We identify a hitherto uncharacterized protein factor that we term UBP (ucm-binding protein) that interacts sequence-specifically with the ucm and determine the structure of the protein both in isolation and when bound to DNA. UBP is a highly abundant protein, and we reveal that it plays a role akin to bacterial nucleoid-associated proteins with over 300 binding sites on the Sulfolobus chromosome. Importantly, UBP interacts with the N-terminal domains of MCM. Taken together, our data provide evidence that UBP functions as a general nucleoid-associated protein that plays a key role in facilitating the egress of the MCM replicative helicase from DNA replication origins.

Next, we solved the structure of UBP bound to DNA containing a ucm site to 1.8 Å resolution. We attempted crystallization with a range of sizes of DNA molecule; the only construct that yielded crystal formation was a 12 nt duplex DNA. Significantly, and in contrast to the homodimeric free protein, UBP binds DNA as a monomer. The interaction with DNA is principally via the major groove and is mediated by two sets of beta-hairpins within the structure, one corresponding to the stirrup loops in the free protein and the other being a part of the 5-beta-strand sheet to which the C-terminal beta strand contributes. Of the three lysine residues in the stirrup loop, K63 makes base-specific contacts in the protein-DNA co-crystal structure. The DNA structure remains close to standard B-form but with a widening of the minor groove to 8 Å at the center of the molecule. Notably, the beta-strand that undergoes the intermonomer strand swap in the DNA-free dimer is now observed to fold back to form an analogous interaction in cis. Furthermore, the interprotomer Y100—F13 π-stacking interaction switches from an offset sandwich orientation in the dimer to a T-shaped interaction in the snapped-back cis configuration of the C-terminal beta strand in the DNA-bound monomer. In contrast to IHF and Fis, although a modest widening of the minor groove is seen, UBP does not introduce any discernible bending of DNA in our protein-DNA co-crystal structure. However, our demonstration that UBP binds the ucm as a monomer suggests this is not the case.

>[2x]MIVMRVKVNEKQFDMIIDKLKLMVYEYNTKIKEYGVYLKPYHIVYKNSKRYIYIGKYWYKLEKIGGKLKWIYLGKTKPIQNMPNPPQIPESTIIKEDNEYIVDEKILYDLE>[2x]TDKLTSLRQYTTVVADTGDIAAMKLY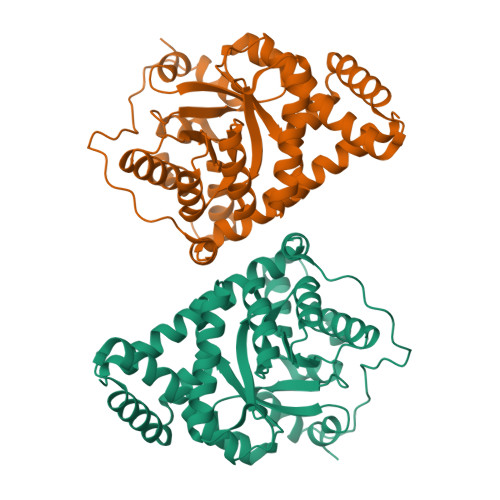QPQDATTAPSLILNAAQIPEYRKLIDDAVAWAKQQSNDRAQQIVDATDKLAVNIGLEILKLVPGRISTEVDARLSYDTEASIAKAKRLIKLYNDAGISNDRILIKLASTWQGIRAAEQLEKEGINCNLTLLFSFAQARACAEAGVFLISPFVGRILDWYKANTDKKEYAPAEDPGVVSVSEIYQYYKEHGYETVVMGASFRNIGEILELAGCDRLTIAPALLKELAESEGAIERKLSYTGEVKARPARITESEFLWQHNQDPMAVDKLAEGIRKFAIDQEKLEKMIGDLL>GSHNMAEMVETVCGPVPVEQLGKTLIHEHFLFGYPGFQGDVTRGTFREDESLRVAVEAAEKMKRHGIQTVVDPTPNDCGRNPAFLRRVAEETGLNIICATGYYYNGEGAPPYFQFRRLLGTAEDDIYDMFMAELTEGIADTGIKAGVIKLASSKGRITEYEKMFFRAAARAQKETGAVIITHTQEGTMGPEQAAYLLEHGADPKKIVIGHMCGNTDPDYHRKTLAYGVYIAFDRFGIQGMVGAPTDEERVRTLLALLRDGYEKQI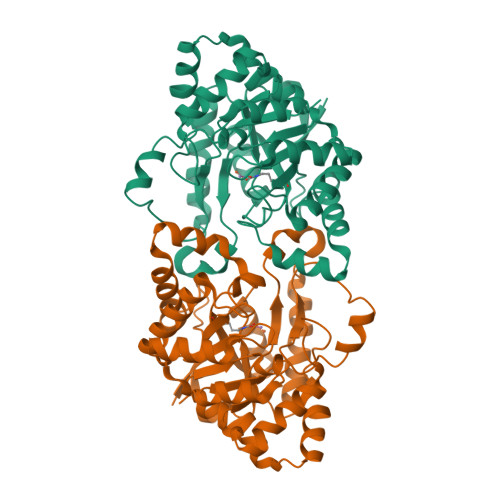MLSHDTVNVWLGRPFTLPEPFAEMMKNWHVEHLFVNIIPALKNEGIRDEVLEQMFIGNPAALFSA[2x]[4-(phenylmethyl)piperidin-1-yl]-[1-(5-pyrrol-1-yl-1,3,4-thiadiazol-2-yl)piperidin-4-yl]methanone 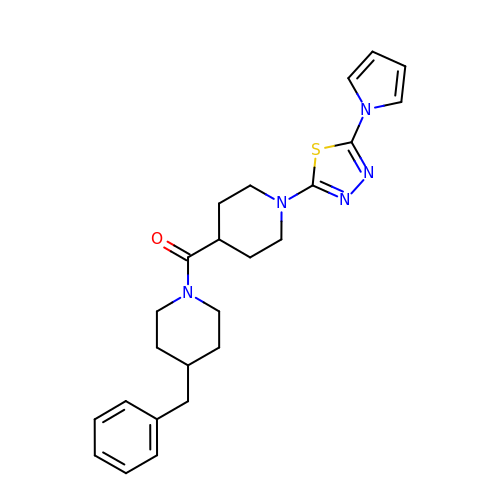| C24 H29 N5 O S | QREVWNVSFCZWGU-UHFFFAOYSA-N antabactin | C34 H35 F N6 O4 | 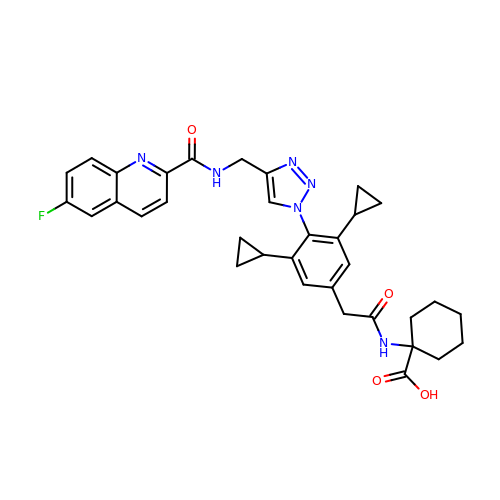RNZLLYIHGGOVPO-UHFFFAOYSA-N> PLQEMLAAPSSFKKSHVLSVTQFTRADLHLLFQIAQEMRLGVQREGVLDILRGKVLCTLFYEPSTRTSASFDAAMQRLGGRTIPIQTSTSSVQKGETLQDTLRTLANYSDAIVLRHPDEKCVD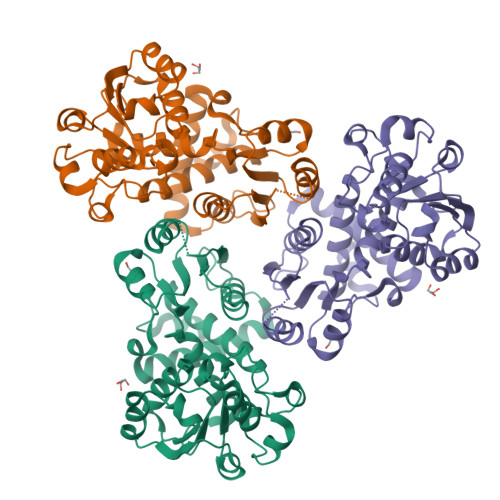VAKKYCPVPVINGGNGSKEHPTQAFLDLFTIREELGTMQGLTITFVGDLLYGRPVHSLVYLLRHYQVKVQLVSPKALRLPPAVRQQLVDAGQLLCESEALTPEILGRTDVLYCTRVQKERFPSLAEFEAVKDSYRIDYSTLKYAKPTTVVMHPLPRNEEVAEEVDFDQRAAYFRQMRYGLYCRMALLALVMS CRISPR–Cas adaptive immune systems capture DNA fragments from invading mobile genetic elements and integrate them into the host genome to provide a template for RNA-guided immunity. Here we reconstitute CRISPR sequence capture, processing and integration by a naturally occurring Megasphaera NM10-related Cas2 and DEDDh fusion protein (Cas2/DEDDh) in complex with Cas1 (Cas1–Cas2/DEDDh). The natural Cas1–Cas2/exonuclease fusion (trimmer-integrase) catalyses coordinated DNA capture, trimming and integration. The Megasphaera Cas1–Cas2 retains the canonical heterohexameric architecture, with two Cas1 dimers (denoted Cas1 and Cas1′, a or b subunit) bridged by a central Cas2 dimer.

Aiming to visualize DEDDh trimming and conformational changes in Cas1, we used cryo-EM to characterize Cas1–Cas2/DEDDh in complex with a DNA half-site analogue containing phosphorothioate linkages at the PAM positions. Isolation and refinement of particle clusters representing maxima of the reaction coordinate gave linear and bent reconstructions at resolutions of 4.1 Å and 3.9 Å, respectively. The DEDDh domain was visible only in the linear conformation. In the linear structure, a Cas1b′ C-terminal loop (Leu279 to Ser293) rich in charged residues is positioned near to the major groove adjacent to the second integration target site. The corresponding density is absent in the 3.1 Å half-site and 2.9 Å prespacer-bound structures, indicating that this loop participates in engagement with the CRISPR repeat on the PAM side. A C-terminal cap, which follows the C-terminal loop, protects the PAM and adjacent nucleotides from trimming by DEDDh. Notably, the DEDDh domain was visible in the linear structure, but on the non-PAM side of the complex, where no overhang trimming occurs. The exonuclease sits in a cavity formed by the interface of the CRISPR repeat DNA, Cas1a/b′ and Cas2, where it appears to contact the repeat DNA backbone and the N terminus of Cas1b. These interactions may beneficially constrain bending of the second integration target site or prevent trans activity.

>MPMTVITLKNVPQSLRGDLTRWMQEIATGVYVGNFNSRIREYLWRRVQETMGAGEASMCFAARNELGYDFLTENASRSVIDYDGLPLIFIPKE[2x];>[4x]MAGPIIAGKSESSELPRVEDRATFIYIEHAKINRVDSAVTVAEAKGVVRIPAAMIGVLLLGPGTDISHRAVELLGDTGTALVWVGEQGVRYYASGRALARSTRFLVKQAELVTNERSRLRVARRMYQMRFPTEDVSKLTMQQLRSHEGARVRRKYRELSKKYNVPWKKRVYNPDDFAGGDPINQALSAAHVALYGLVHSVVAALGLSPGLGFVHTGHDRSFIYDVADLYKAEITVPIAFAVAAEAEEGQDIGQLARLRTRDAFVDGKILKRMVKDLQTLLEIPEEGQIEAEPLSLWDDKEKLVPYGVNYSE;> IRYVVIDIETDGKDAKRNHILEIGAIRCEDGKETHFTALISGDAVPPSITKLTGITATLLQKEGQEEKKVLTAFREFIGDDDLVGYHVSFDIEFLRQAFKKYGLGYLKNKTHDLLRIVKKEQLFQADYKLETSLQSYGIHKKVPHRALGDAELVKCLAKKLNKF Clostridial collagenases are among the most efficient enzymes to degrade by far the most predominant protein in the biosphere. Clostridia employ collagenases for nutrition (e.g. saprophytic strains) and host colonization (1–3). They are large multidomain proteins of ∼115 kDa belonging to the gluzincin superfamily of metalloproteases. Here we present the crystal structures of the peptidase domains of ColH and ColT and the collagenase unit of ColG in the presence and absence of the peptidic inhibitor isoamylphosphonyl-Gly-Pro-Ala bound to the active site.

The peptidase domains of ColH (Q46085; Pro330–Gly721; 46 kDa) and ColT (Q899Y1; Asp340–Lys731; 46 kDa) showed sequence identities of 56 and 55% and sequence similarities of 71 and 74%, respectively. The stabilizing interactions of the helper subdomain with the upper segment and, to a lower extent, with the lower catalytic segment are reflected by their contact areas of 1060 and 418 Å2 for ColG, 1046 and 347 Å2 for ColH, and 955 and 503 Å2 for ColT. The upper and lower segments form a 959-, 1115-, and 1359 Å2 contact area, respectively. Consequently, the contact area between the upper and lower catalytic subdomains is larger by 42% in ColT than in ColG. Similarly, the lower catalytic subdomain has more than 20% stabilizing interactions with the helper domain, together suggesting a considerably more rigid quaternary arrangement within the peptidase in ColT as compared with ColG and also ColH. This difference might point toward different substrate specificities in these enzymes; alternatively, the PKD domain(s) present in ColG/H might compensate for the additional quaternary stabilization found in ColT. As evidenced by the comparison of Ca2+-unloaded (ColG) and -loaded (ColH/T) crystal structures, the liganding glutamate side chain undergoes a marked rearrangement upon Ca2+ binding that allows Ca2+ coordination. Due to its location between the two catalytic helices, calcium binding braces the upper and lower half-domains of the peptidase and stabilizes thereby the zinc coordination. Notably, the peptidase domain of ColG from C. histolyticum showed a higher structural similarity to ColT from C. tetani than to ColH from C. histolyticum.

>GGTDINKLIEEGKKHYLPKTYTFDNGKIIIKAGDKVEESKIQKLYWASKEVKSQFHRIIGNDKPLEVGNADDILTIVIYNNPEEYKLNKTLYGYSVDNGGIYIEGIGTFFTYERTPQESIYSLEELFRHEFTHYLQGRYLIPGLFNKGDFYKGNNGRITWFEEGSAEFFAGSTRTSVLPRKSMVGGLSKNPKERFNADKLLHSKYSDGWDFYKYGYAFSDYMYNNNKKLFSDLVSTMKNNDVKGYEALIEESSKDSKINKDYEYHMENLVNNYDNYTIPLVSDDYMKQYDNKSLHEIKSDIEKAMDVKNSQITKESSQYFDTYNLKATYTLSSNKGEISNWNYMNNKINEALNKLDNLSWGGYKTVTAYFSNPRLNSNNEVVYDIVFHGLLSHN[2x]Here, inspired by natural and re-engineered protein–peptide systems, we set out to design proteins made out of repeating units that bind peptides with repeating sequences, with a one-to-one correspondence between the repeat units of the protein and those of the peptide. We use geometric hashing to identify protein backbones and peptide-docking arrangements that are compatible with bidentate hydrogen bonds between the side chains of the protein and the peptide backbone. We design repeat proteins to bind to six different tripeptide-repeat sequences in polyproline II conformations. The proteins are hyperstable and bind to four to six tandem repeats of their tripeptide targets with nanomolar to picomolar affinities in vitro and in living cells.

Reasoning that proline-containing peptides would incur a lower entropic cost upon binding than non-proline-containing peptides, we decided to start our experimental characterization with designs containing at least one proline residue; in most of these designs, the peptide backbone is in or near the polyproline II portion of the Ramachandran map. For the polyproline helix, there are roughly three residues per turn, and, probably because of this, we obtained more designs that target three-residue than two-residue proline-containing repeat units. Crystal structures reveal repeating interactions between protein and peptide interactions as designed, including ladders of hydrogen bonds from protein side chains to peptide backbones. Our results show that by matching superhelical parameters between repeating-protein and repeating-peptide conformations, and incorporating specific hydrogen-bonding and hydrophobic interactions between matched protein and peptide repeats, we can now design modular proteins that bind to extended peptides with high affinity and specificity.

> DREEAAFLAASILIQHAHEQGKDDRELEKILEIAIRILEKNGVDREEAAFLAASILIQHAHEQGKDDRELEKILEIAIRILEKNGVDREEAAFLAASILIQHAHEQGKDDRELEKILEIAIRILEKNGVDREEAAFLAASILIQHAHEQGKDDRELEKILEIAIRILEKNGV;> LRPLRPLRPLRP(2R,2'R)-3,3'-oxydipropane-1,2-diol 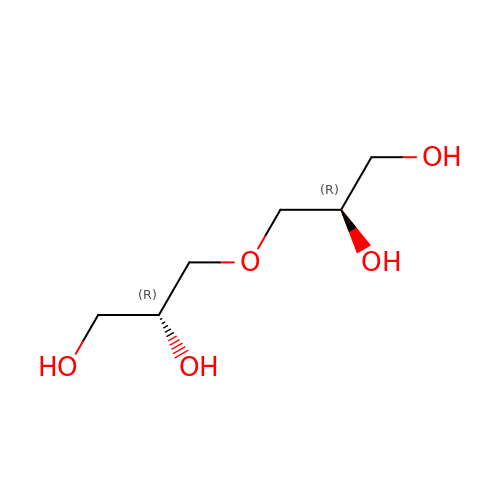| C6 H14 O5 | GPLRAVKSCUXZTP-PHDIDXHHSA-N>[3x]SIIQVTFIAGRTELQKERLIAALTDAAVDTVGIERAEVRVILKDIPNTDYGIAGQTARSLGRGVDRHGRAPGGS;>PNIEMFVVEGYSDQQKEALVGALTQATVEAIGAPI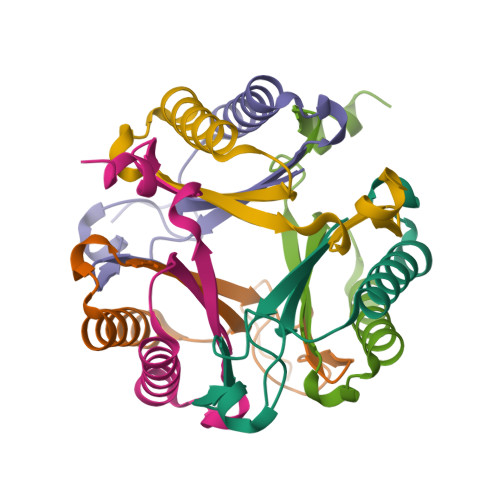DSVRVWLTEVPATQFGIGGKTVAAIAAGQE[3x]> RLSGYCGSPWRVIGYHVVVWMMAGIPLLLFRWKPLWGVRLRLRPCNLAHAETLVIEIRDKEDSSWQLFTVQVQTEAIGEGSLEPSPQSQAEDGRSQAAVGAVPEGAWKDTAQLHKSEEAKRVLRYYLFQGQRYIWIETQQAFYQVSLLDHGRSCDDVHRSRHGLSLQDQMVRKAIYGPNVISIPVKSYPQLLVDEALNPYYGFQAFSIALWLADHYYWYALCIFLISSISICLSLYKTRKQSQTLRDMVKLSMRVCVCRPGGEEEWVDSSELVPGDCLVLPQEGGLMPCDAALVAGECMVNESSLTGESIPVLKTALPEGLGPYCAETHRRHTLFCGTLILQARAYVGPHVLAVVTRTGFCTAKGGLVSSILHPRPINFKFYKHSMKFVAALSVLALLGTIYSIFILYRNRVPLNEIVIRALDLVTVVVPPALPAAMTVCTLYAQSRLRRQGIFCIHPLRINLGGKLQLVCFDKTGTLTEDGLDVMGVVPLKGQAFLPLVPEPRRLPVGPLLRALATCHALSRLQDTPVGDPMDLKMVESTGWVLEEEPAADSAFGTQVLAVMRPPLWEPQLQAMEEPPVPVSVLHRFPFSSALQRMSVVVAWPGATQPEAYVKGSPELVAGLCNPETVPTDFAQMLQSYTAAGYRVVALASKPLPTVPSLEAAQQLTRDTVEGDLSLLGLLVMRNLLKPQTTPVIQALRRTRIRAVMVTGDNLQTAVTVARGCGMVAPQEHLIIVHATHPERGQPASLEFLPMESPTAVNGVKDPDQAASYTVEPDPRSRHLALSGPTFGIIVKHFPKLLPKVLVQGTVFARMAPEQKTELVCELQKLQYCVGMCGDGANDCGALKAADVGISLSQAEASVVSPFTSSMASIECVPMVIREGRCSLDTSFSVFKYMALYSLTQFISVLILYTINTNLGDLQFLAIDLVITTTVAVLMSRTGPALVLGRVRPPGALLSVPVLSSLLLQMVLVTGVQLGGYFLTLAQPWFVPLNRTVAAPDNLPNYENTVVFSLSSFQYLILAAAVSKGAPFRRPLYTNVPFLVALALLSSVLVGLVLVPGLLQGPLALRNITDTGFKLLLLGLVTLNFVGAFMLESVLDQCLPACLRRLRPKRASKKRFKQLERELAEQ

ATP13A2, which is mutated in juvenile-onset Parkinson’s disease and autosomal recessive spastic paraplegia 78, is a transporter with a critical role in balancing the polyamine concentration between the lysosome and the cytosol. The overall structure of hATP13A2 has a canonical P-type ATPase architecture, with the cytosolic A domain linking to TM1 and TM2 domains, and the N and P domains sitting on the TM4 and TM5. The P-type ATPases transport substrates by coupling ATP hydrolysis with protein phosphorylation states and adopting a series of intermediate states, consisting of E1, E1-ATP, E1P-ADP, E1P, E2P, E2-Pi, and E2, in a process known as the Post-Albers reaction. Here, we report seven cryo-EM structures of hATP13A2 in six intermediate states, importantly including the putative E2 and E1-like states, thereby providing a nearly complete atomic-level conformational cycle spanning the Post-Albers reaction process.

Adenine nucleotides (AMP-PCP or ADP) or phosphate analogs (BeF3− or AlF4−) were used to stabilize hATP13A2 in the E1-ATP or E1P/E2P intermediate states. However, in the structures obtained after incubation with BeF3− and AlF4−, no significant difference was observed. By comparing with known E2P structures, we suggest that both BeF3− and AlF4− incubated structures are in the same E2P state. Accordingly, we found a polyamine entrance binding pocket positioned in the endo-/lysosomal luminal leaflet with an outward-opening architecture in the E2P structure of hATP13A2. Spatially, the entrance site (denoted as Site1) located among TM1, TM2, TM4a, TM5, and TM6, had a chalk-shaped architecture open to the luminal side where substrates were captured. The chalk-shaped EM density, in conjunction with the results of a liquid chromatography-tandem mass spectrometry (LC-MS/MS) experiment, suggested the presence of a linear endogenous spermine (SPM) substrate. There are also several negatively charged residues, such as D254, E456, and D960, located near the entrance to the chalk-shaped pocket, which may be important for the recruitment of positively charged polyamines into Site1. The gating feature of Site1 was further supported by all-atom explicit solvent MD simulations of hATP13A2 in the E2P state, which revealed that, despite being deeply buried in the membrane bilayer, Site1 could be hydrated. In E2P state, conformational rearrangements in the cytosolic domains and transmembrane regions induce the opening of the entrance pocket Site1, and the negatively charged amino acids are enabled to recruit positively charged polyamines (shown in green). The low pH environment of the lysosome may favor the recruitment of polyamines from the luminal side to the negatively charged entrance Site1 in the E2P state.>MTPFFSSLKDNRIFQFTVVSIIILNAVLIGATTYELDPLFLETIHLLDYGITIFFVIEILIRFIGEKQKADFFKSGWNIFDTVIVAISLIPIPNNSSFLVLRLLRIFRVLRLISVIPELKQIIEAILESVRRVFFVSLLL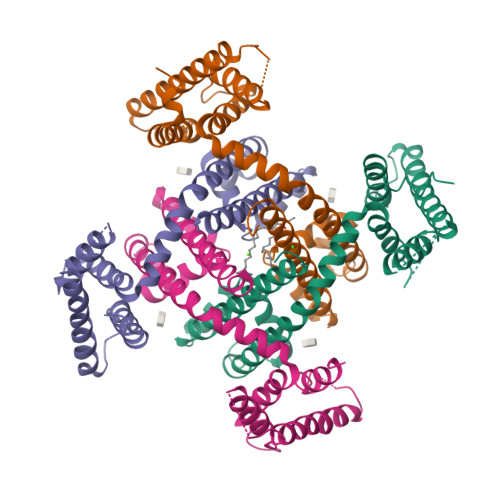FIILYIYATMGAILFGNDDPSRWGDLGISLITLFQVLTLSSWETVMLPMQEIYWWSWVYFFSFIIICSITILNLVIAILVDVVIQKKLE[4x]>[4x]MNTDRYDSLTEVEVEGLSYLYNFADGHAYHDINEHYVDIINNLQRYWQEGKDHSIPDMEKAFKNQFAELIDSSTLHSTNH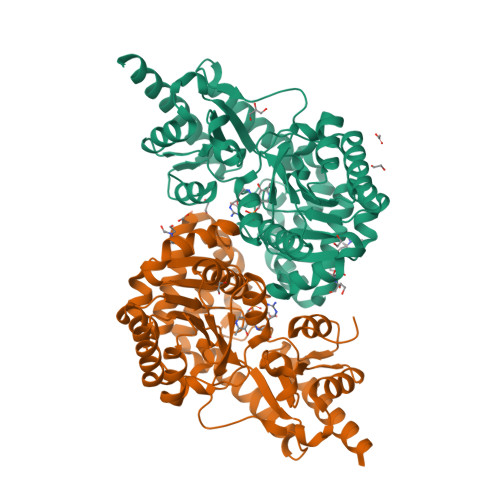FSVCPTASNSIDIVAAWLHKENKRTALIEPAFDNLYLLLKRRGVDISAFDELALKNEHQLAQIVSSGDIDALFLVNPNNPTGLEMTESEFVYLVEQCKAHNITILLDRTFRIYGKTNFDDYQILEQSGIDYVVIEDTGKTWPTQDLKISLMVYSEAISSTMRLLYEEIFLCSSNFALALLKQFVAVTAKFGVDATIKNEVRRRSETINDALAGTGLKVFDNDEKCQLPLCWIDISATGYDDVSFAARLKEHDIAVLPGRFFYWNSKSQHTQFIRVSLMKPDAEFYEGIGKLKEAVTRILEKLEHHHHHH> RIIGGSDADIKNFPWQVFFDNPWAGGALINEYWVLTAAHVVEGNREPTMYVGSTSVQTSRLAKSKMLTPEHVFIHPGWKLLEVPEGRTNFDNDIALVRLKDPVKMGPTVSPICLPGTSSDYNLMDGDLGLISGWGRTEKRDRAVRLKAARLPVAPLRKCKEVKVEKPTADAEAYVFTPNMICAGGEKGMDSCKGDSGGAFAVQDPNDKTKFYAAGLVSWGPQCGTYGLYTRVKNYVDWIMKTMQENSTPRED;> LRYHGDPMPCPKEDTPNSVWEPAKAKYVFRDVVQITCLDGFEVVEGRVGATSFYSTCQSNGKWSNSKLKCQPVDCGIPESIENGKVEDPESTLFGSVIRYTCEEPYYYMENGGGGEYHCAGNGSWVNEVLGPELPKCVPVCGVPREPFEEKQ;> AHHHHHHTSGDDDDKAKKKLPKCQKQEDCGSWDLKCNNVTKKCECRNQVCGRGCPKERYQRDKYGCRKCLCKGCDGFKCRLGCTYGFKTDKKGCEAFCTCNTKETAC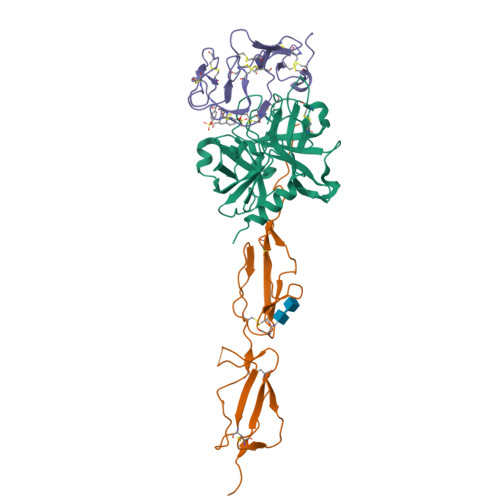VNIWCTDPYKCNPESGRCEDPNEEYEYDYE>SNAMASNDVVVLQDSTFEQEVLKSDTPVLVDFWAVWCGPCKAIAPVVDDLAARYKGKLKVAKMDVDQHQGVPQQYGIRSIPTLLVF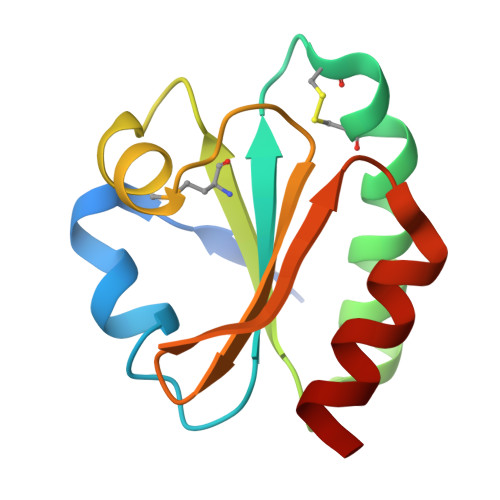KGGRVVDTVIGADKTRLEDSVKKAIG[2x]>[3x]MHHHHHHMLEAKFEEASLFKRIIDGFKDCVQLVNFQCKEDGIIAQAVDDSRVLLVSLEIGVEAFQEYRCDHPVTLGMDLTSLSKILRCGNNTDTLTLIADNTPDSIILLFEDTKKDRIAEYSLKLMDIDADFLKIEELQYDSTLSLPSSEFSKIVRDLSQLSDSINIMITKETIKFVADGDIGSGSVIIKPFVDMEHPETSIKLEMDQPVDLTFGAKYLLDIIKGSSLSDRVGIRLS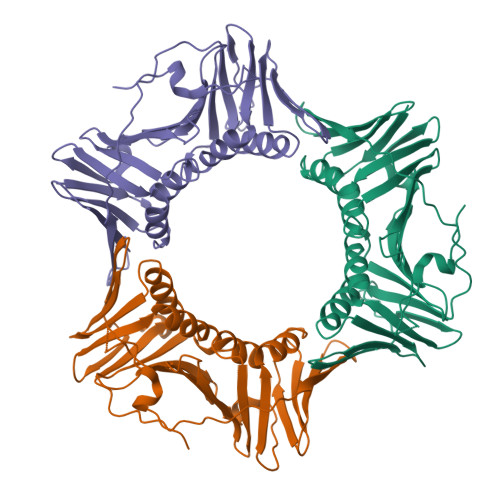SEAPALFQFDLKSGFLQFFLAPKFNDEEGGSGGAKERAQSRIGNFFKKLSDS> GPPVVEEDDVVGFDDEAQTVIDRLLEGSGDLEVIPVVGMPGLGKTTLATKIFKHPKIEYEFFTRLWLYVSQSYKTRELYLNIISKFTGNTKHCRDMSEKDLALKVQEILEEGGKYLIVLDDVWSTDAWDRIKIAFPKNDKGNRVLLTTRDHRVARYCNRSPHDLKFLTDEESWILLEKRAFHKAKCLPELETNGKSIARKCKGLPLAIVVIAGALIGKSKTIKEWEQVDQSVGEHFINRDQPNSCDKLVRMSYDVLPYDWKACFLYFGTFPRGYLIPARKLIRLWIAEGFIQYRGDLSPECKAEEYLNELVNRNLVMVMQRTVDGQIKTCRVHDMLYEFCWQEATTE

The majority of these plant intracellular receptors belong to the nucleotide-binding leucine-rich repeat (NLR) protein family, similar to those involved in certain animal cell-death or innate immune responses. Plant NLRs share a common architecture with animal NLRs, containing nucleotide binding (NB) and Leucine-rich repeat (LRR) domains, but can be further classified into CNLs and TNLs, dependent on whether they have an N-terminal coiled-coil (CC) domain or N-terminal toll/interleukin-1 receptor (TIR) domain. The N-terminal CC or TIR domains are typically described as required for downstream signalling following perception of pathogens, the LRR is implicated in auto-inhibition and/or effector detection, and the central NB-ARC domain is posited as a regulatory domain, acting as a “switch” that determines whether the protein is in an active or inactive state. Here we characterise the NB-ARC domain from the tomato NLR NRC1, which we have expressed and purified from both bacterial (E. coli) and insect (Sf9) cell culture.

Isomorphous native crystals of the NRC1 NB-ARC domain were generated, and X-ray data collected to 2.5 Å resolution. Iterative manual rebuilding and refinement resulted in a final structure consisting of 252 of a total 346 residues present in the expressed protein construct. Several regions of the protein could not be modelled due to discontinuous electron density, including much of the ARC1 subdomain, and the solvent-exposed ɑ-helices of the NB domain. Submission of this model to the DALI server returns APAF-1 as the major structural homologue, despite sharing little (24%) sequence identity. The electron density within the nucleotide-binding pocket of the NRC1 NB-ARC domain, and the surrounding regions, was well resolved and allowed us to unambiguously position a molecule of ADP, and the side-chains of interacting residues. These included lysine 191 of the Walker A (P-loop) motif, aspartate 267 and 268 of the Walker B motifs, and histidine 480 of the MHD motif. Using PDBe PISA, we defined a network of side-chain and main-chain interactions between the bound ADP and the protein. This network includes lysine 191 (P-loop motif) and histidine 480 (MHD motif), as well as hydrophobic interactions from the GLPL motif, and other surrounding residues, resulting in a ligand-binding pocket with over 90% of the ADP surface area buried within the protein. The result of this extensive interaction surface is a binding pocket partially occluded by the positioning of the ARC2 subdomain, suggesting structural rearrangements will be required to allow nucleotide release. The NRC1 NB-ARC domain structure in the vicinity of the bound ADP is unambiguously defined by the electron density, as are the relative orientations of the NB, ARC1 and ARC2 domains. Here, the NRC1 NB-ARC domain behaves as a monomer in solution and packing in the crystal lattice does not suggest a functionally relevant oligomerisation state.>MNTVRSEKDSMGAIDVPADKLWGAQTQRSLEHFRISTEKMPTSLIHALALTKRAAAKVNEDLGLLSEEKASAIRQAADEVLAGQHDDEFPLAIWQTGSGTQSNMNMNEVLANRASELLGGVRGMERKVHPNDDVNKSQSSNDVFPTAMHVAALLALRKQLIPQLKTLTQTLNEKSRAFADIVKIGRTHLQDATPLTLGQEISGWVAMLEHNLKHIEYSLPHVAELALGGTAVGTGLNTHPEYARRVADELAVITCAPFVTAPNKFEALATCDALVQAHGALKGLAASLMKIANDVRWLASGPRCGIGEISIPENEPGSSIMPGKVNPTQCEALTMLCCQVMGNDVAINMGGASGNFELNVFRPMVIHNFLQSVRLLADGMESFNKHCAVGIEPNRERINQLLNESLMLVTALNTHIGYDKAAEIAKKAHKEGLTLKAAALALGYLSEAEFDSWVRPEQMVGSMKAGRHHHHH[2x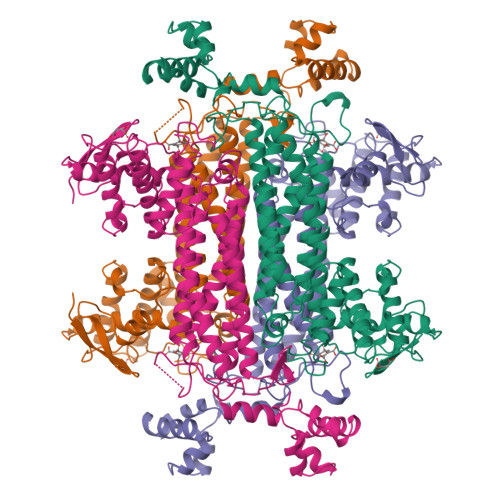]> MGNRGMEDLIPLVNRLQDAFSAIGQNADLDLPQIAVVGGQSAGKSSVLENFVGRDFLPRGSGIVTRRPLVLQLVNATTEYAEFLHCKGKKFTDFEEVRLEIEAETDRVTGTNKGISPVPINLRVYSPHVLNLTLVDLPGMTKVPVGDQPPDIEFQIRDMLMQFVTKENCLILAVSPANSDLANSDALKVAKEVDPQGQRTIGVITKLDLMDEGTDARDVLENKLLPLRRGYIGVVNRSQKDIDGKKDITAALAAERKFFLSHPSYRHLADRMGTPYLQKVLNQQLTNHIRDTLPGLRNKLQSQLLSIEKEVEE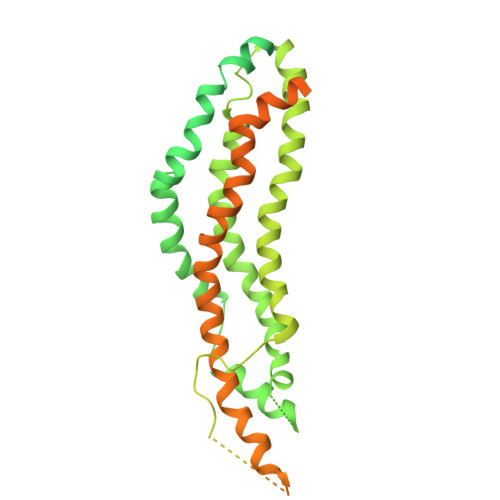YKNFRPDDPARKTKALLQMVQQFAVDFEKRIEGSGDQIDTYELSGGARINRIFHERFPFELVKMEFDEKELRREISYAIKNIHGIRTGLFTPDMAFETIVKKQVKKIREPCLKCVDMVISELISTVRQCTKKLQQYPRLREEMERIVTTHIREREGRTKEQVMLLIDIELAYMNTNHEDFIGFANAQQRSNQMNKKKTSGNQDEILVIRKGWLTINNIGIMKGGSKEYWFVLTAENLSWYKDDEEKEKKYMLSVDNLKLRDVEKGFMSSKHIFALFNTEQRNVYKDYRQLELACETQEEVDSWKASFLRAGVYPERVGDKEKASETEENGSDSFMHSMDPQLERQVETIRNLVDSYMAIVNKTVRDLMPKTIMHLMINNTKEFIFSELLANLYSCGDQNTLMEESAEQAQRRDEMLRMYHALKEALSIIGDINTTTVSTPMPPPVDDSWLQVQSVPAGRRSPTSSPTPQRRAPAVPPARPGSRGPAPGPPPAGSALGGAPPVPSRPGASPDPFGPPPQVPSRPNRAPPGVPSRSGQASPSRPESPRPPFDL>[3x]TTCTGCTGCTGAA;> TTCT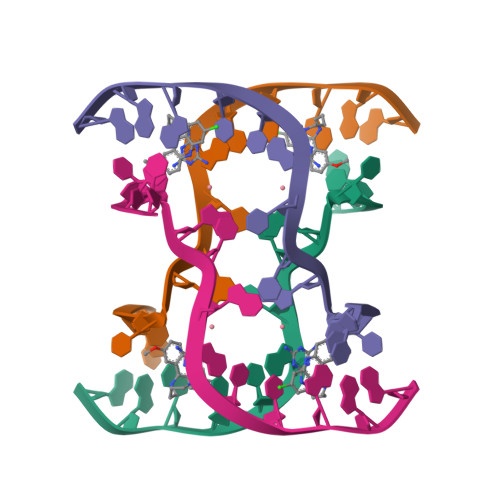GCAGCTGAA>[2x]SNAMETKTVAITMGDPAGIGPEIIVKALSEDGLNGAPLVVIGCLATLKRLQAKGITPNVELRAIERVAEARFAPGIIHVIDEPLAQPEALEAGKVQAQAGDLAYRCVKRATELALRGDVQAI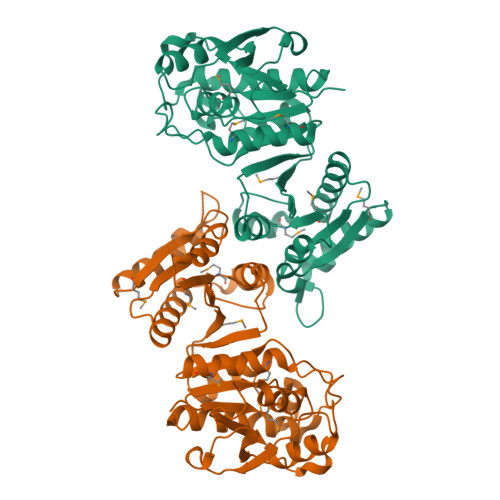ATAPLNKEALHLAGHNYPGHTELLATLTHSRDYAMVLYTDKLKVIHVSTHIALRKFLDTLSTARVETVIGIADTFLKRVGYVKPRIAVAGVNPHAGENGLFGDEETRILTPAITDARAKGMDVYGPCPPDTVFLQAYEGQYDMVVAMYHDQGHIPLKLLGFYDGVNITAGLPFIRTSADHGTAFDIAWTGKAKSESMAVSIKLAMQLA> MSGGDGRGHNTGAHSTSGNINGGPTGIGVSGGASDGSGWSSENNPWGGGSGSGIHWGGGSGRGNGGGNGNSGGGSGTGGNLSAVAAPVAFGFPALSTPGAGGLAVSISASELSAAIAGIIAKLKKVNLKFTPFGVVLSSLIPSEIAKDDPNMMSKIVTSLPADDITESPVSSLPLDKATVNVNVRVVDDVKDERQNISVVSGVPMSVPVVDAKPTERPGVFTASIPGAPVLNISVNDSTPAVQTLSPGVTNNTDKDVRPAGFTQGGNTRDAVIRFPKDSGHNAVYVSVSDVLSPDQVKQRQDEENRRQQEWDATHPVEAAERNCERARAELNQANEDVARNQERQAKAVQVYNSRKSELDAANKTLADAIAEIKQFNRFAHDPMAGGHRMWQMAGLKAQRAQTDVNNKQAAFDAAAKEKSDADAALSAAQERRKQKENKEKDAKDKCAMESKRNKPGKAT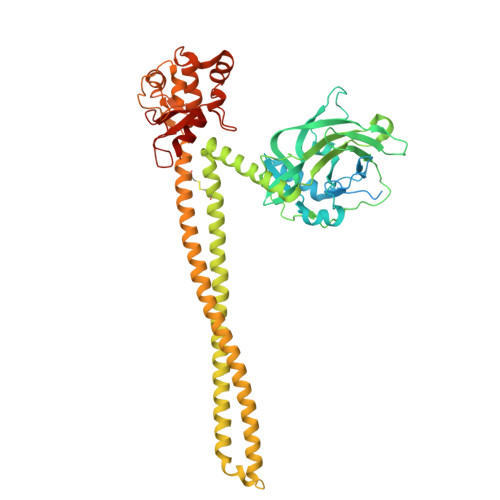GKGKPVGDKWLDDAGKDSGAPIPDRIADKLRDKEFKSFDDFRKAVWEEVSKDPELSKNLNPSNKSSVSKGYSPFTPKNQQVGGRKVYELHHDKPISQGGEVYDMDNIRVTTPKRHIDIHRGK> IKGGLFADIASHPWQAAIFAKHRRSPGERFLCGGILISSCWILSAAHCFQERFPPHHLTVILGRTYRVVPGEEEQKFEVEKYIVHKEFDDDTYDNDIALLQLKSDSSRCAQESSVVRTVCLPPADLQLPDWTECELSGYGKHEALSPFYSERLKEAHVRLYPSSRCTSQHLLNRTVTDNMLCAGDTRSGGPQANLHDACQGDSGGPLVCLNDGRMTLVGII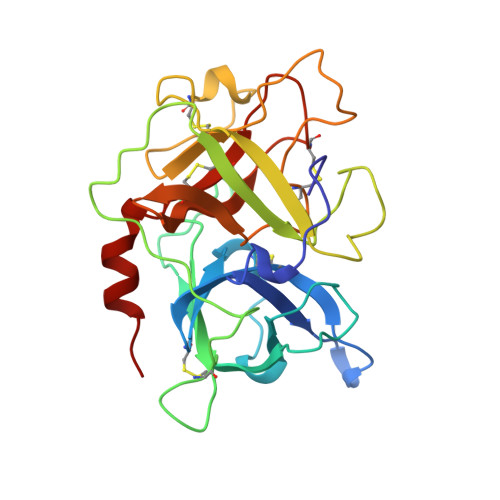SWGLGCGQKDVPGVYTKVTNYLDWIRDNMRP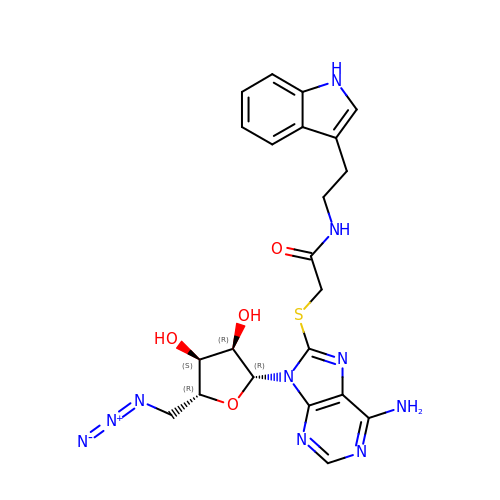5'-azido-5'-deoxy-8-[(2-{[2-(1H-indol-3-yl)ethyl]amino}-2-oxoethyl)sulfanyl]adenosine | C22 H24 N10 O4 S | NZVSVIHQZMZCNV-HAXDFEGKSA-N N-(2,3-dimethylphenyl)-2-(morpholin-4-yl)acetamide 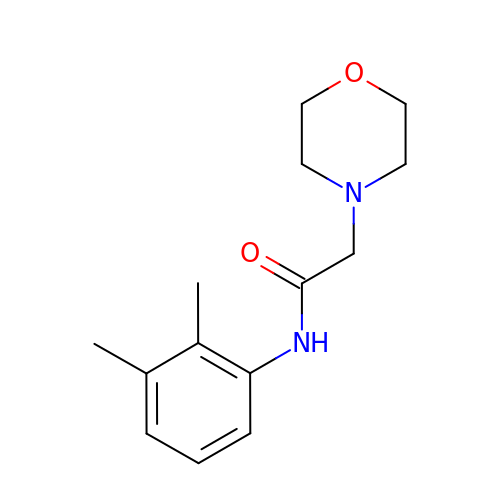| C14 H20 N2 O2 | PPTFUQPLPCCALB-UHFFFAOYSA-N> GKAE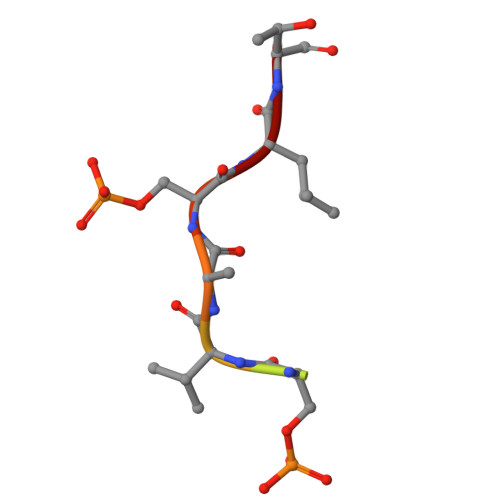SVASLT>[4x]MKSQSIMSVERSAETSLTLEIPTSPLIIKITQQERNILSNVGNLLVKAFGNYENPDYIASLHLHAFQLLPERITRILSQFGSDFSAEQYGAIVFQGLIEVDQDDLGPTPPNWQGADYGKLNKYGFICSLLHGAVPSKPVQYYAQRKG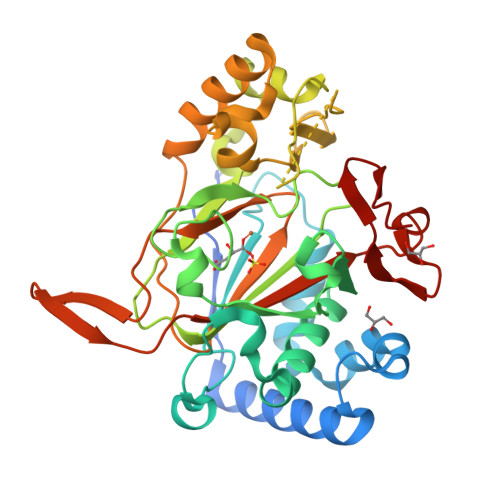GGLLHAVIPDEKMAATQTGSGSKTDLFVHTEDAFLSNQADFLSFLYLRNEERVPSTLYSIRSHGKMNPVMKKLFEPIYQCPKDANYNDEDVANSGPTASVLYGNRELPFIRFDAAEQIFNENAGQTSEALGNLMDFWDEAKTLINSDYIPNSGDLIFVNNHLCAHGRSAFIAGQRIENGEIIKCERRQMLRMMSKTSLIHIRSVTRTDDPYFIMEEHLGKIFDLD> SPRWQETAYVLGNYKTEPCKKPPRLCRQGYACPYYHNSKDRRRSPR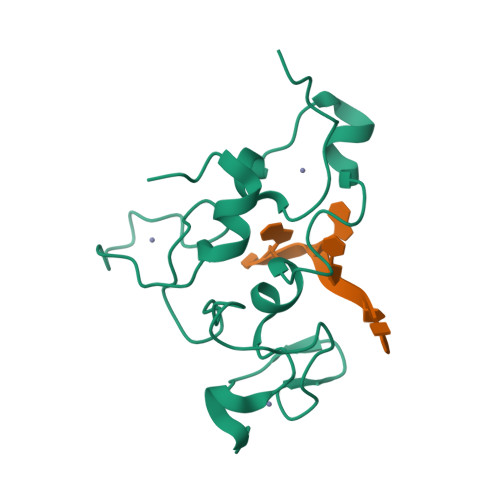KHKYRSSPCPNVKHGDEWGDPGKCENGDACQYCHTRTEQQFHPEIYKSTKCNDMQQAGSCPRGPFCAFAHIEPPPLSDDVQPSSAVS> XSRVAELANAVVSNADQKDLLRMSWGVLSVDMEGTGLMLMANLFKTSPSAKGKFARLGDVSAGK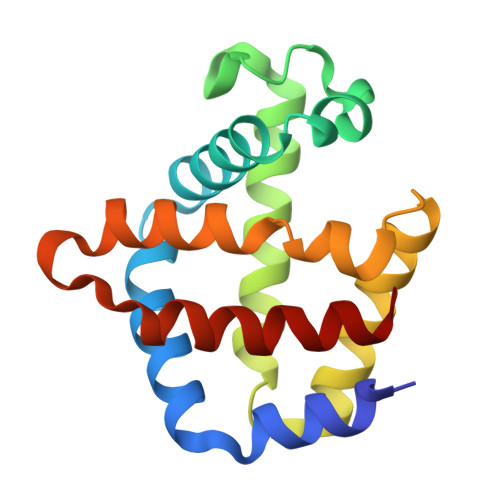DNSKLRGHSITLMYALQNFVDALDDVERLKCVVEKFAVNHINRQISADEFGEIVGPLRQTLKARMGNYFDEDTVAAWASLVAVVQAAL>SAVRLVPHRAIYDLTLDRADEKSGISGLTGRMVYEFNGSACEGYTTNFRFVTRVDMDEQPQRVTDQQTTTFEDADGKDFRFVNKTFVDKELVKEVRGDAKLEDGKTVVKLSKPKENTLDLKGTQFPTRHMEELIGKAEAGQKFYQTTLFDASEDADRVVATTVVVGKQQAVPDDETKVMGKFSKDQVWPVTIAYFDDKEQQDGMPIYRINFKLYRNGITRDMTMDYGDFSMRGKLVKL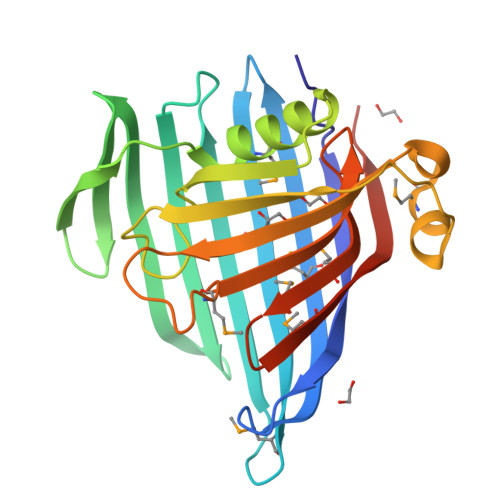DIYDTGKNKTGCSK[4x]> GPHLICQSGDVLSARYEIVDTLGEGAFGKVVECIDHKAGGRHVAVKIVKNVDRYCEAARSE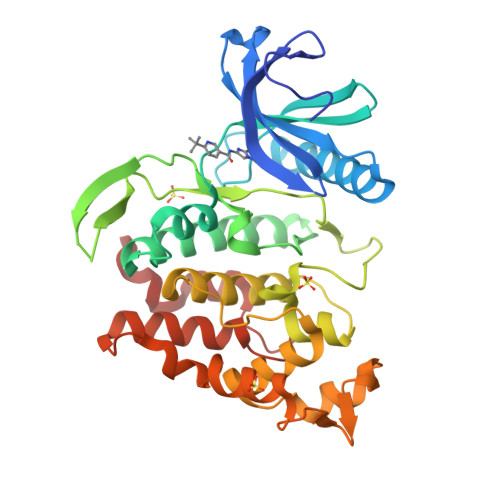IQVLEHLNTTDPNSTFRCVQMLEWFEHHGHICIVFELLGLSTYDFIKENGFLPFRLDHIRKMAYQICKSVNFLHSNKLTHTDLKPENILFVQSDYTEAYNPKIKRDERTLINPDIKVVDFGSATYDDEHHSTLVSTRHYRAPEVILALGWSQPCDVWSIGCILIEYYLGFTVFPTHDSKEHLAMMERILGPLPKHMIQKTRKRKYFHHDRLDWDEHSSAGRYVSRRCKPLKEFMLSQDVEHERLFDLIQKMLEYDPAKRITLREALKHPFFDLLKKSI> MAIRNFVFKISNQIQNLAAKRSLAYLNQIDSQSVPSRATINMKDQVTQMQREIDNMANVIRAQIPDEDRAEFEILKKYYVTGQHDSLVDPQDVLLQLDRIQVL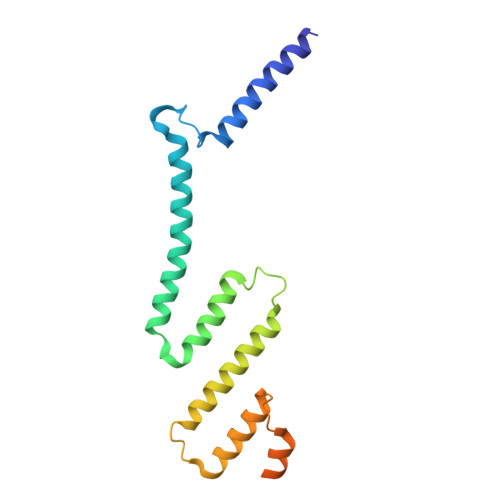KNLKMIELNEEAYDPELVRLEKLKARVLLEEEGALLEYAHFISKRPYNKPYEKWGVSEEHVKQQILG>[4x]MAPKKVLLALTSYNDVFYSDGAKTGVFVVEALHPFNTFRKEGFEVDFVSETGKFGWDEHSLAKDFLNGQDETDFKNK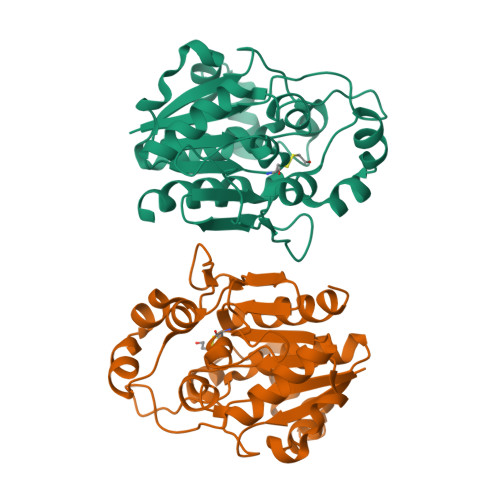DSDFNKTLAKIKTPKEVNADDYQIFFASAGHGTLFDYPKAKDLQDIASEIYANGGVVAAVCHGPAIFDGLTDKKTGRPLIEGKSITGFTDVGETILGVDSILKAKNLATVEDVAKKYGAKYLAPVGPWDDYSITDGRLVTGVNPASAHSTAVRSIDALKN>MFKDGSLIPYLTAGDPDKQSTLNFLLALDEYAGAIELGIPFSDPIADGKTIQESHYRALKNGFKLREAFWIVKEFRRHSSTPIVLMTYYNPIYRAGVRNFLAEAKASGVAGILVVDLPVFHAKEFTEIAREEGIKTVFLAAPNTPDERLKVIDDMTTG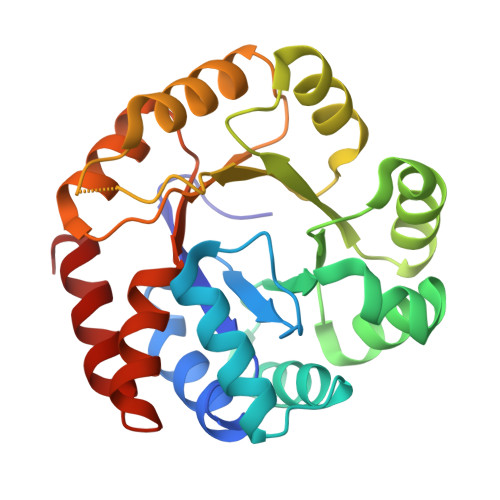FVYLVSLYGTTGAREEIPKTAYDLLRRAKRICRNKVAVGFGVSKREHVVSLLKEGANGVVVGSALVKIIGEKGREATEFLKKKVEELLGI[2x]>SADVAGAVIDGAGLGFDVLKTVLEALGNVKRKIAVGIDNESGKTWTAMNTYFRSGTSD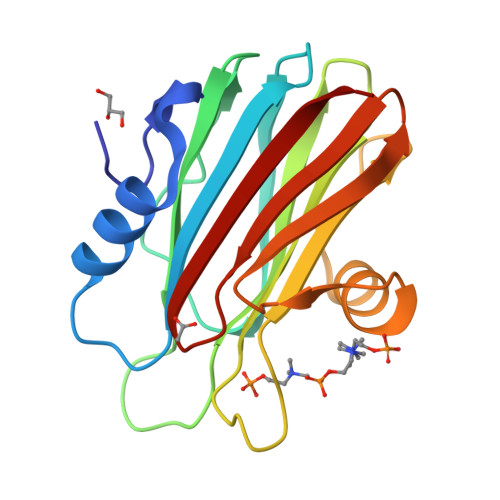IVLPHKVAHGKALLYNGQKNRGPVATGVVGVIAYSMSDGNTLAVLFSVPYDYNWYSNWWNVRVYKGQKRADQRMYEELYYHRSPFRGDNGWHSRGLGYGLKSRGFMNSSGHAILEIHVTKA[2x]> TVDDILEQVGESGWFQKQAFLILCLLSAAFAPICVGIVFLGFTPDHHCQSPGVAELSQRCGWSPAEELNYTVPGLGPAGEAFLGQCRRYEVDWNQSALSCVDPLASLATNRSHLPLGPCQDGWVYDTPGSSIVTEFNLVCADSWKLDLFQSCLNAGFLFGSLGVGYFADRFGRKLCLLGTVLVNAVSGVLMAFSPNYMSMLLFRLLQGLVSKGNWMAGYTLITEFVGSGSRRTVAIMYQMAFTVGLVALTGLAYALPHWRWLQLAVSLPTFLFLLYYWCVPESPRWLLSQKRNTEAIKIMDHIAQKNGKLPPADLKMLSLEEDVTEKLSPSFADLFRTPRLRKRTFILMYLWFTDSVLYQGLILHMGATSGNLYLDFLYSALVEIPGAFIALITIDRVGRIYPMAMSNLLAGAACLVMIFISPDLHWLNIIIMCVGRMGITIAIQMICLVNAELYPTFVRNLGVMVCSSLCDIGGIITPFIVFRLREVWQALPLILFAVLGLLAAGVTLLLPETKGVALPETMKDAENLG

The human organic cation transporter 1 (hOCT1), also known as SLC22A1, is integral to hepatic uptake of structurally diversified endogenous and exogenous organic cations, influencing both metabolism and drug pharmacokinetics. hOCT1 has been implicated in the therapeutic dynamics of many drugs, making interactions with hOCT1 a key consideration in novel drug development and drug–drug interactions. As part of the major facilitator superfamily (MFS), hOCT1 operates on an alternating access mechanism, allowing substrate-binding sites to be exposed alternately to either side of the membrane via transporter conformational changes. Each hOCT1 transport cycle involves transitioning from the outward open to the outward occluded, then inward occluded, and finally the inward open states. The protein can be divided into several different regions, with the N-terminal domain (NTD) comprising transmembrane helices 1–6 (TMs 1–6), and the C-terminal domain (CTD), consisting of transmembrane segments 7–12 (TMs 7-12).

In the case of hOCT1-metformin in DDM micelles, we successfully delineated structures in three conformations: outward open (hOCT1-M1), outward occluded (hOCT1-M2), and inward occluded (hOCT1-M3), at resolutions ranging from 3.8 to 4.1 Å. The shift from the outward open to the occluded state is characterized by the movement of the extracellular termini of the CTD helices, with the intracellular portions of these helices exhibiting minimal displacement. This results in channel narrowing, as helices TM9, TM10, TM11, TM12 converge towards the cavity, followed by TM7 approaching the central cavity by moving ~ 1.5 Å. During transition from the outward occluded state to the inward occluded state, both the extracellular and intracellular ends of the CTD helices rearrange significantly.> TMAHHHHHHHHHGIEGRMSQDTEVDMKEVELNELEPEKQPMNAASGAAMSLAGAEKNGLVKIKVAEDEAEAAAAAKFTGLSKEELLKVAGSPGWVRTRWALLLLFWLGWLGMLAGAVVIIVRAPRCRELPAQKWWHTGALYRIGDLQAFQGHGAGNLAGLKGRLDYLSSLKVKGLVLGPIHKNQKDDVAQTDLLQIDPNFGSKEDFDSLLQSAKKKSIRVILDLTPNYRGENSWFSTQVDTVATKVKDALEFWLQAGVDGFQVRDIENLKDASSFLAEWQNITKGFSEDRLLIAGTNSSDLQQILSLLESNKDLLLTSSYLSDSGSTGEHTKSLVTQYLNATGNRWCSWSLSQARLLTSFLPAQLLRLYQLMLFTLPGTPVFSYGDEIGLDAAALPGQPMEAPVMLWDESSFPDIPGAVSANMTVKGQSEDPGSLLSLFRRLSDQRSKERSLLHGDFHAFSAGPGLFSYIRHWDQNERFLVVLNFGDVGLSAGLQASDLPASASLPAKADLLLSTQPGREEGSPLELERLKLEPHEGLLLRFPYAA;> MAWSHPQFEKIEGRMEEGARHRNNTEKKHPGGGESDASPEAGSGGGGVALKKEIGLVSACGIIVGNIIGSGIFVSPKGVLENAGSVGLALIVWIVTGFITVVGALCYAELGVTIPKSGGDYSYVKDIFGGLAGFLRLWIAVLVIYPTNQAVIALTFSNYVLQPLFPTCFPPESGLRLLAAICLLLLTWVNCSSVRWATRVQDIFTAGKLLALALIIIMGIVQICKGEYFWLEPKNAFENFQEPDIGLVALAFLQGSFAYGGWNFLNYVTEELVDPYKNLPRAIFISIPLVTFVYVFANVAYVTAMSPQELLASNAVAVTFGEKLLGVMAWIMPISVALSTFGGVNGSLFTSSRLFFAGAREGHLPSVLAMIHVKRCTPIPALLFTCISTLLMLVTSDMYTLINYVGFINYLFYGVTVAGQIVLRWKKPDIPRPIKINLLFPIIYLLFWAFLLVFSLWSEPVV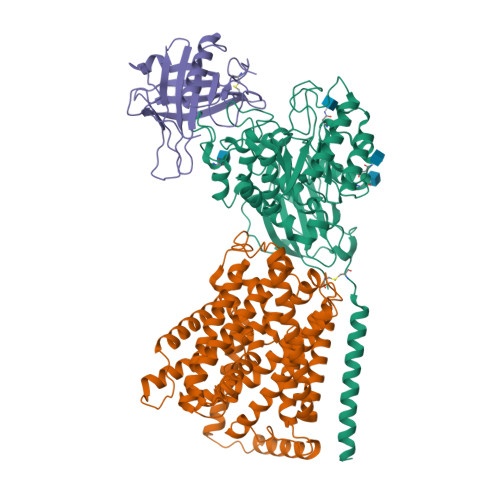CGIGLAIMLTGVPVYFLGVYWQHKPKCFSDFIELLTLVSQKMCVVVYPEVERGSGTEEANEDMEEQQQPMYQPTPTKDKDVAGQPQP;> QDSTSDLIPAPPLSKVPLQQNFQDNQFHGKWYVVGRAGNTGLREDKDPGKMFATIYELKEDKSYNVTYVWSGQKKCMYSIVTFVPGSQPGEFTLGNIKSAPGRTSWLVRVVSTNYNQHAMVFFKSVTQNREGFAITLYGRTKELTSELKENFIRFSKSLGLPENHIVFPVPIDQCIDGSAWSHPQFEK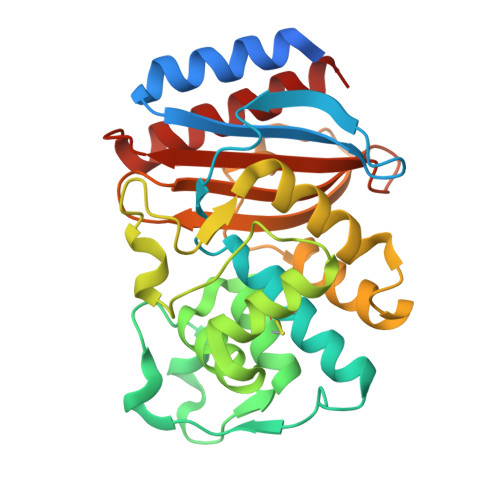> MSIQHFRVALIPFFAAFCLPVFAHPETLVKVKDAEDQLGARVGYIELDLNSGKILESFRPEERFPMMGTFKVLLCGAVLSRIDAGQEQLGRRIHYSQNDLVEYSPVTEKHLTDGMTVRELCSAAITMSDNTAANLLLTTIGGPKELTAFLHNMGDHVTRLDRWEPELNEAIPNDERDTTMPVAMATTLRKLLTGELLTLASRQQLIDWMEADKVAGPLLRSALPAGWFIADKSGAGERGSRGIIAALGPDGKPSRIVVIYTTGSQATMDERNRQIAEIGASLIKHW The use of Glc in all these pathways depends on its activation to UDP-glucose (UDP-Glc) in a reaction catalyzed by UDP-glucose pyrophosphorylase (UGP; EC 2.7.7.9). With the exception of plants and certain protozoa, where a second enzyme with broader substrate specificity can form UDP-Glc4567, UGP is the only enzyme capable of producing UDP-Glc from glucose-1-phosphate (Glc-1-P) and uridine triphosphate (UTP). The available crystal structures revealed eukaryotic UGPs to comprise a structurally conserved central catalytic domain with Rossmann-like α/β/α sandwich fold (reviewed in Kleczkowski et al.), flanked by a flexible N-terminal domain with low conservation at primary sequence level and regulatory function in S. cerevisiae, as well as a C-terminal β-helix domain171819. In the fungal and animal kingdom, the complexity of UGP function is further increased by their octameric organization, which was shown for human UGP (hUGP) to be essential for enzymatic activity.

We thereby resolved the UDP-Glc complexed conformation of the full-length hUGP isoform 1, which represents the first product-bound crystal structure of an octameric UGP, and thus enabled us to identify the binding mode of UDP-Glc and to discover an intermolecular mechanism - we termed it interlock - that stabilizes the sugar-binding region. The asymmetric unit of the crystal contained four hUGP1 molecules (chains A, B, C and D) which formed a non-crystallographic cyclic C4 tetramer. The bound UDP-Glc enabled the detailed analysis of the active site, which is located in a deep groove at the center of the catalytic domain (purple) and consists of a twisted eight-stranded β-sheet (white arrows) flanked by α-helices, a structural motif characteristic for nucleotide binding domains. Electron density analysis revealed the binding mode of the product UDP-Glc in the active site of hUGP1, where it is coordinated by the NB-loop, parts of the eight-stranded β-sheet and other residues of the catalytic domain. The phosphate groups of UDP-Glc are coordinated by the active site residues K127, H223 and N251. Compared to the apo-structure, the side chain of H223 is rotated by 90° in the UDP-Glc state and thus reaches a position which allows formation of an H-bond with the β-phosphate moiety. Movements of the N- and C-terminal domains toward the active site upon UDP-Glc binding (closing of the structure) resulted in a slightly more compact geometry with a deeper active site cleft. A more prominent rearrangement was observed in the SB-loop region, which undergoes a considerable tilt. R287 of the SB-loop of one subunit (A′, light green) forms H-bonds with D456 at the base of the C-terminal β-helix domain of the neighboring subunit (A, dark purple), to which it is connected side-by-side; likewise, R287 (A) interacts with D456 (A′).

>[4x]MASWSHPQFEKGALVPRGSSRFVQDLSKAMSQDGASQFQEVIRQELELSVKKELEKILTTASSHEFEHTKKDLDGFRKLFHRFLQEKGPSVDWGKIQRPPEDSIQPYEKIKARGLPDNISSVLNKLVVVKLNGGLGTSMGCKGPKSLIGVRNENTFLDLTVQQIEHLNKTYNTDVPLVLMNSFNTDEDTKKILQKYNHCRVKIYTFNQSRYPRINKESLLPVAKDVSYSGENTEAWYPPGHGDIYASFYNSGLLDTFIGEGKEYIFVSNIDNLGATVDLYILNHLMNPPNGKRCEFVMEVTNKTRADVKGGTLTQYEGKLRLVEIAQVPKAHVDEFKSVSKFKIFNTNNLWISLAAVKRLQEQNAIDMEIIVNAKTLDGGLNVIQLETAVGAAIKSFENSLGINVPRSRFLPVKTTSDLLLVMSNLYSLNAGSLTMSEKREFPTVPLVKLGSSFTKVQDYLRRFESIPDMLELDHLTVSGDVTFGKNVSLKGTVIIIANHGDRIDIPPGAVLENKIVSGNLRILDH> KPKNKDKDKKVPEPDNKKKKPKKEEEQKWKWWEEERYPEGIKWKFLEHKGPVFAPPYEPLPENVKFYYDGKVMKLSPKAEEVATFFAKMLDHEYTTKEIFRKNFFKDWRKEMTNEEKNIITNLSKCDFTQMSQYFKAQTEARKQMSKEEKLKIKEENEKLLKEYGFCIMDNHKERIANFKIEPPGLFRGRGNHPKMGMLKRRIMPEDIIINCSKDAKVPSPPPGHKWKEVRHDNKVTWLVSWTENIQGSIKYIMLNPSSRIKGEKDWQKYETARRLKKCVDKIRNQYREDWKSKEMKVRQRAVALYFIDKLALRAGNEKEEGETADTVGCCSLRVEHINLHPELDGQEYVVEFDFLGKDSIRYYNK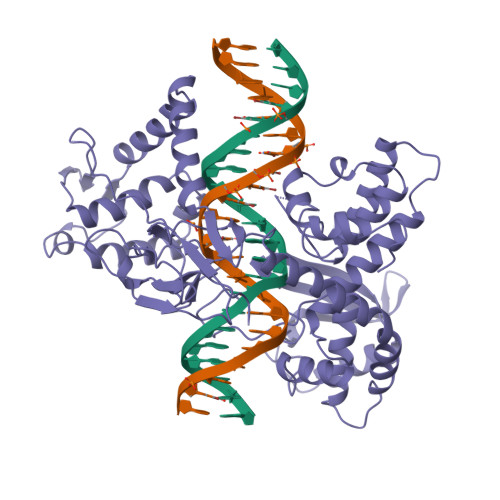VPVEKRVFKNLQLFMENKQPEDDLFDRLNTGILNKHLQDLMEGLTAKVFRTYNASITLQQQLKELTAPDENIPAKILSYNRANRAVAILCNHQRAPPKTFEKSMMNLQTKIDAKKEQLADARRDLKSAKADAKVMKDAKTKKVVESKKKAVQRLEEQLMKLEVQATDREENKQIALGTSKLNFLDPRITVAWCKKWGVPIEKIYNKTQREKFAWAIDMADEDYEF> MRGSHHHHHHGMASELALMNSLTTAAGATLAATDQYRPAFHYTAERNWLNDPNGLVYLNGTYHLFYQHNPFGADWGNMSWGHATSRDLLHWDEQPVAIPCDEHEAIFSGSAVFDQHNTSGLGTAANPPLVAIYTSAYSDAAPLPGRQAQSLAYSLDEGRTWTKYHGNPVLDRASADFRDPKVFWYDGGAGSYWVMVAVEAVQRQVVLYKSADLKAWEHLSTFGPANATGGVWECPDLFELPVDGNPEDNRWVLIVNINPGGIAGGSAGQYFVGEFDGVAFHSGSTVTEGLQKDSSRMREYGWLDWGRDYYAAVSFSNVPDGRRIMIGWMNNWDYARETPTGGWRSAMSLPREVSLTRVDGKVMLRQQAIDPLPERETGHVRLGPQPLASG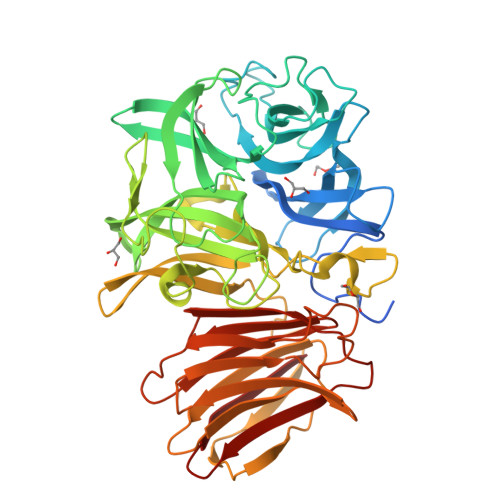VLDVPAAASVARIDVELEPGAAAGVGLVLRAGDDERTVLRYDTSDGMLRLDRRESGQVAFHETFPSIEAMAVPLQGGRLRLRVYLDRCSVEVFAQDGLATLTDLVFPGEASTGLAIFAEGEGAHLVVLDVVGR>[2x]MSYYHHHHHHLESTSLYKKAGLDYDIPTTENLYFQGMNTLREVVPVPREQLARSRVLVVGDVMLDRYWFGNVDRISPEAPVPVVHVQRQEERLGGAANVARNAVTLGGQAGLLCVVGCDEPGERIVELLGSSGVTPHLERDPALPTTIKLRVLARQQQL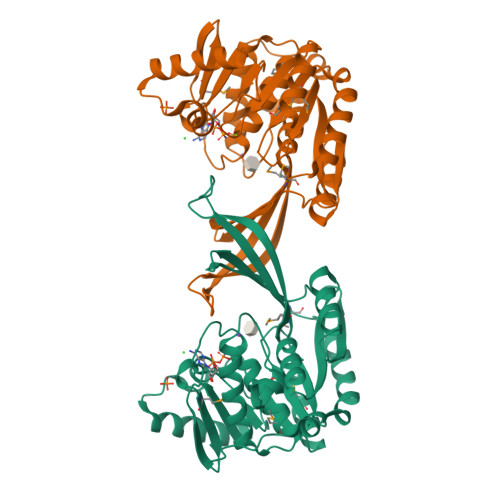LRVDFEAMPTHEVLLAGLARFDVLLPQHDVVLMSDYAKGGLTHVTTMIEKARAAGKAVLVDPKGDDWARYRGASLITPNRAELREVVGQWKSEDDLRARVANLRAELDIDALLLTRSEEGMTLFSAGGELHAPALAREVFDVSGAGDTVIATVATMLGAGVPLVDAVVLANRAAGIVVGKLGTATVDYDELFH> MECFVPLRCDLD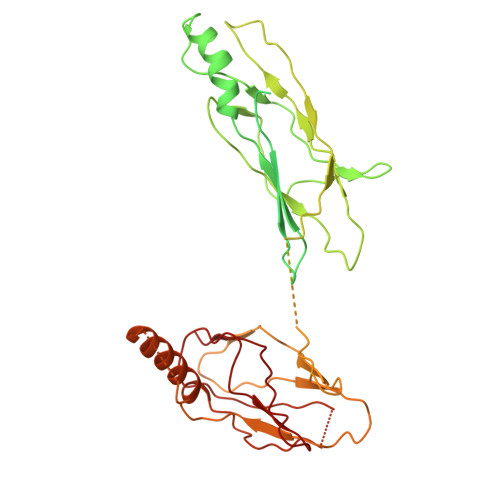GSNIEQLRQSHLSRKFIIFDEQLNLWLWFQGNSQENKRFVLQNMIILINEAQVTRTSTIDDYFTQVENNENLWRLKNDCCSKILFKSNVVMNNGYNNQIKFVFEYKSVDANFNNQDSLQDPQAKYTLDKYSSEEILPSFEPVYSWSSAATKSSKNTNNHLEKNNRATHRVSSKNSEVHEADVSRNPNTFTLKLQYPIFSLLNMRLRNISLKSEHCILSSLDFQTSKASEQLTKKFIYPQEHNSFLKLNFQEISYKLIDGTSQIELDPICPLKVPLTAFSYDSISATFKLVLLPKSTQPHRVKITLAYELELHPNLKLPVRTSWETEVTLKRSMPISSTSSQYSSNNNNTNHSASFNGAANNVNSGGLANLRLGGVSSSRFSLGAASTTSLVNSKLSNVKFKFINSNIKVIKGEKFTMRLQIINSSSSPLDLVVYYNNTINPIPSANNVRNSNGINNCGMNNGTIPNSPLTLENQYQLHNKYRKIAEGIILLSNDYKIPVVPPRETYFADLRFIGIMSGYYGTLSGLKVLDLNTNELIEVGNGASVLI> GSHMASPTPAPSQSPIRRDAFSIIEAEEYNSTNSSTLQVIGTPNN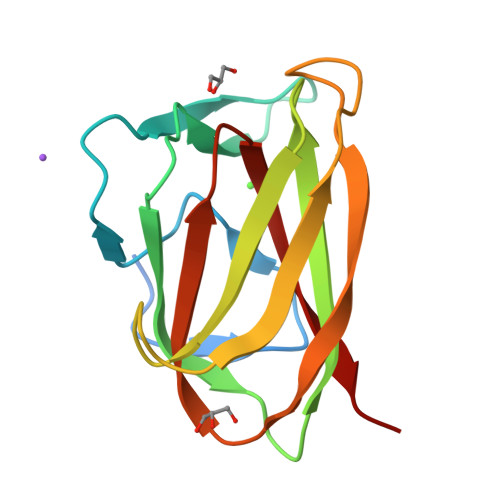GRGIGYIENGNTVTYSNIDFGSGATGFSATVATEVNTSIQIRSDSPTGTLLGTLYVSSTGSWNTYNTVSTNISKITGVHDIVLVFSGPVNVDNFIFSRSS> GKVTFPKMKIPKF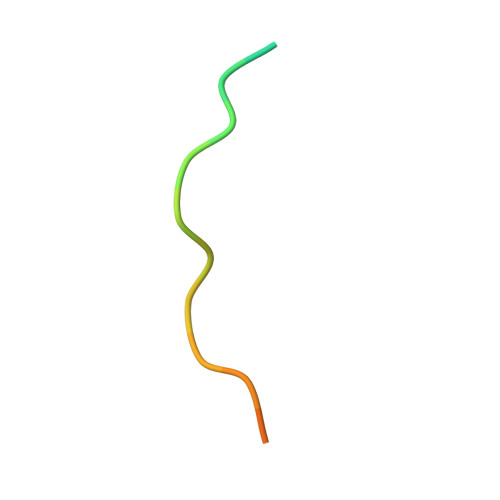TFSGREL> MTVLMRLVASAYSIAQKAGMIVRRVIAEGDLGIVEKTCATDLQTKADRLA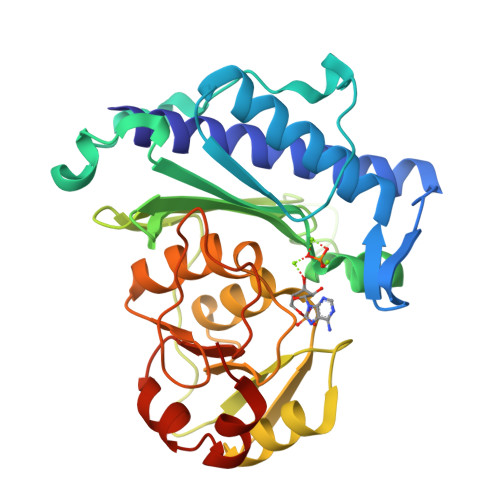QMSICSSLARKFPKLTIIGEEDLPSEEVDQELIEDSQWEEILKQPCPSQYSAIKEEDLVVWVDPLDGTKEYTEGLLDNVTVLIGIAYEGKAIAGVINQPYYNYEAGPDAVLGRTIWGVLGLGAFGFQLKEVPAGKHIITTTRSHSNKLVTDCVAAMNPDAVLRVGGAGNKIIQLIEGKASAYVFASPGCKKWDTCAPEVILHAVGGKLTDIHGNVLQYHKDVKHMNSAGVLATLRNYDYYASRVPESIKNALVPAHHHHHH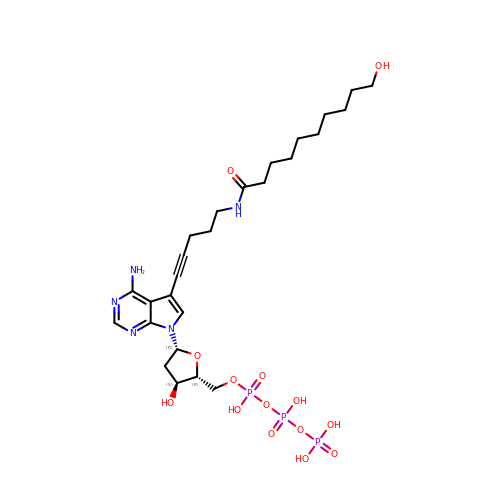7-{2-deoxy-5-O-[(S)-hydroxy{[(S)-hydroxy(phosphonooxy)phosphoryl]oxy}phosphoryl]-beta-D-erythro-pentofuranosyl}-5-{5-[(10-hydroxydecanoyl)amino]pent-1-yn-1-yl}-7H-pyrrolo[2,3-d]pyrimidin-4-amine | C26 H42 N5 O14 P3 | JQTQPUSSMXPQMW-QZNHQXDQSA-N>[2x]MGKAVIAIHGGAGAISRAQMSLQQELRYIEALSAIVETGQKMLEAGESALDVVTEAVRLLEECPLFNAGIGAVFTRDETHELDACVMDGNTLKAGAVAGVSHLRNPVLAARLVMEQSPHVMMIGEGAENFAFARGMERVSPEIFSTSLRYEQLLAARKEGATVLDHSGAPLDEKQKMG;>TVGAVALDLDGNLAAATSTGGMTNKLPYQVGPTPLVGAGCYANNASVAVSCTGTG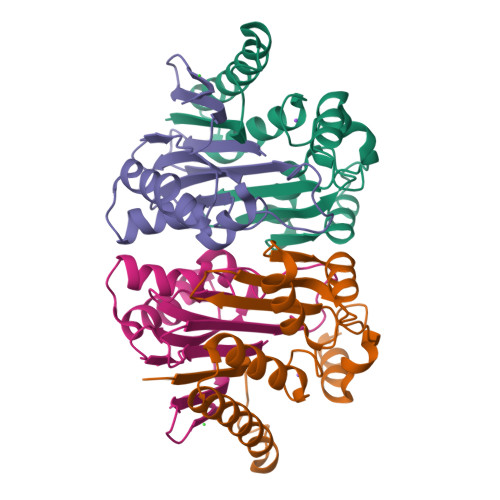EVFIRALAAYDIAALMDYGGLSLAEACERVVMEKLPALGGSGGLIAIDHEGNVALPFNTEGMYRAWGYAGDTPTTGIYREKGDTVATQ[2x]> GEGKEDAF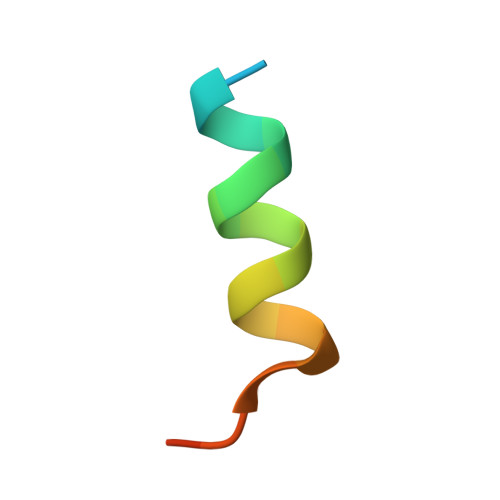SKLKEKFMNELHK> XLASALA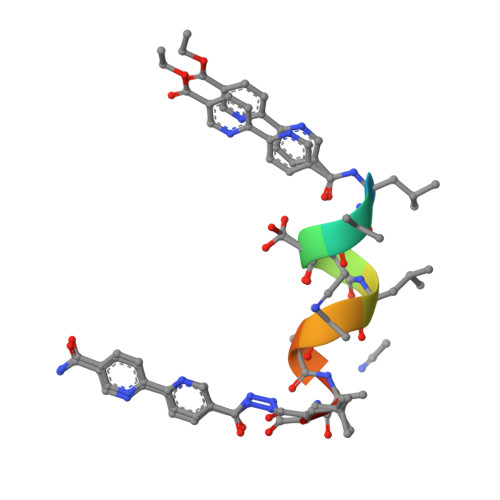QALX>[2x]MKHHHHHHPMTTKQWGITPPISTAPATEQENALNTALINELKNQNLFESPAESEKRVKVLDELQQITTEFVKKVSLAKHMNEKMANEAGGKIFTYGSYRLGVYGPGSDIDTLVVVPKHVSRDNFFQDLEPMLREREEVTDLAAVPDAYVPIIKFKFLGISIDLIFARLSVPRVPRDLELSDNNLLKGVEERCVLSLNGTRVTDQILQLVPNRAVFKHALRAIKFWAQRRAIYANVVGFPGGVAWA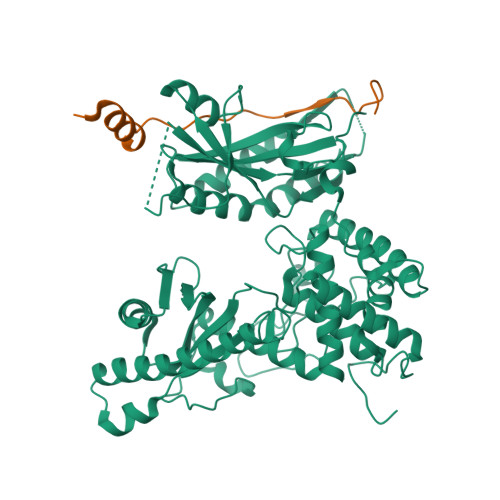MMVARICQLYPNAVSSVIVAKFFRILHQWNWPQPILLKPIEDGPLQVRIWNPKLYPSDKAHRMPIITPAYPSMCATHNITLSTQTIILREMVRAGEIADQIMVKALPWSALFQKHDFFHRYKHYLTITAAAKTAEAQLKWAGLVESKLRHLVTRLELVDAIALAHPFNKGFDKVYNCSSEEEAQQVASGVTLEVAYESTDHEKLANDTVNEEKADNTESKADGSENGEKQIFPVYTTTCYIGLELEKKKGHPIKRLDISWPTQEFYELCKKWDKYDDTLMNVFIKNTKNTALPDEVFEPGEERPKATKKRSTADTAHSTEQLKRQKVSTA;>[2x]GAMGISLPLLKQDDWLSSSKPFGSSTPNVVIEFDSDDDGDDFSNSKIEQSNLEKPPSNSENGGSHHHHHH>EPGRRGSFVEMVDNLRGKSGQGYYVEMTVGSPPQTLNILVDTGSSNFAVGAAPHPFLHRYYQRQLSSTYRDLRKGVYVPYTQGKWEGELGTDLVSIPHGPNVTVRANIAAITESDKFFINGSNWEGILGLAYAEIARPDDSLEPFFDSLVKQTHVPNLFSLQLCGAGFPLNQSEVLASVGGSMIIGGIDHSLYTGSLWYTPIRREWYYEVIIVRVEINGQDLKMDCKEYNYDKSIVDSGTTNLRLPKKVFEAAVKSIKAASSTEKFPDGFWLGEQLVCWQAGTTPWNIFPVISLYLMGEVTNQSFRITILPQQYLRPVED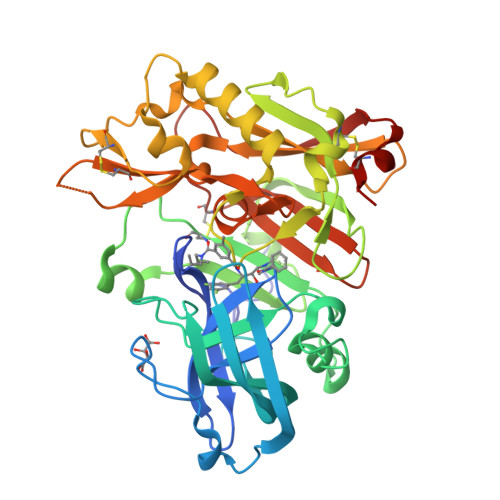VATSQDDCYKFAISQSSTGTVMGAVIMEGFYVVFDRARKRIGFAVSACHVHDEFRTAAVEGPFVTLDMEDCGYNI[2x]>[4x]MAMTLRDMDAVRPVNREAVDRHKARMRDEVRAFRLRE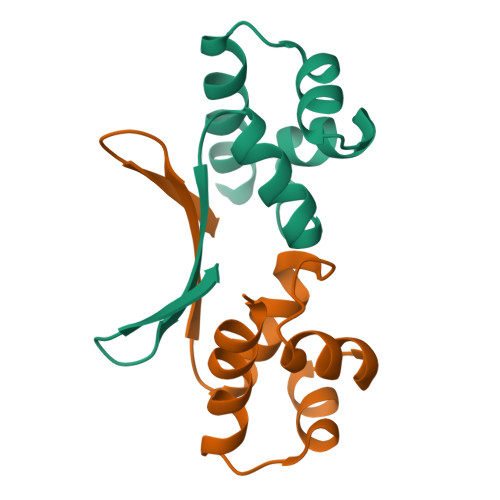LRAAQSLTQVQVAALAHIRQSRVSSIENGDIGSAQVNTLRKYVSALGGELDITVRLGDETFTLA>[2x]ELKFLVVDDNSTMRRIVR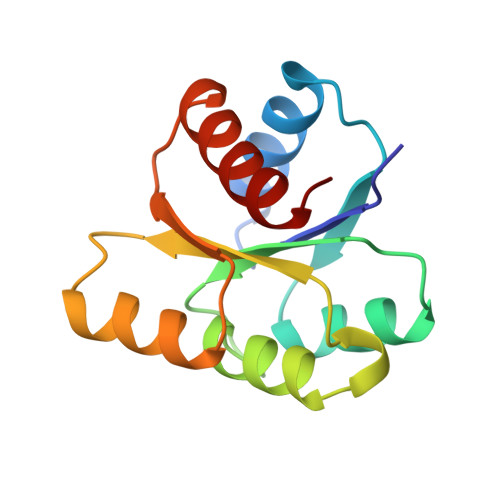NLLKELGFNNVEEAEDGVDALNKLQAGGYGFVISDWNMPNMDGLELLKTIRADGAMSALPVLMTTAEAKKENIIAAAQAGASGYVVKPFTAATLEEKLNKIFEKLGM>[2x]MNAKTDFSGYEVGYDIPALPGMDESEIQTPCLILDLDALER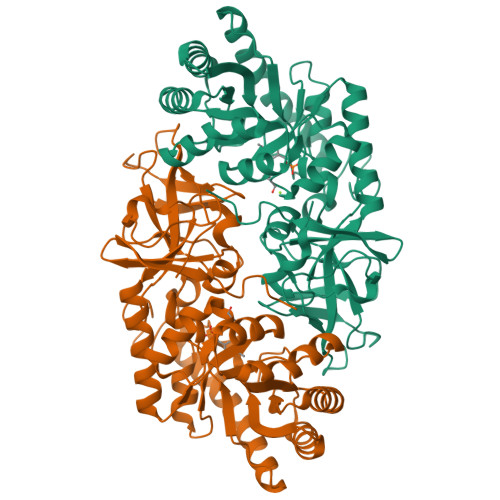NIRKMGDYAKAHGMRHRSHGKMHKSVDVQKLQESLGGSVGVCCQKVSEAEAFARGGIKDVLVTNEVREPAKIDRLARLPKTGATVTVCVDDVQNIADLSAAAQKHGTELGIFVEIDCGAGRCGVTTKEAVVEIAKAAAAAPNLTFKGIQAYQGAMQHMDSFEDRKAKLDAAIAQVKEAVDALEAEGLAPEFVSGGGTGSYYFESNSGIYNELQCGSYAFMDADYGRIHDAEGKRIDQGEWENALFILTSVMSHAKPHLAVVDAGLKAQSVDSGLPFVYGRDDVKYIKCSDEHGVVEDKDGVLKVNDKLRLVPGHCDPTCNVHDWYVGVRNGKVETVWPVSARGKGY> GSADAEYDVVVLGGGPGGYSAAFAAADEGLKVAIVERYKTLGGVCLNVGCIPSKALLHNAAVIDEVRHLAANGIKYPEPELDIDMLRAYKDGVVSRLTGGL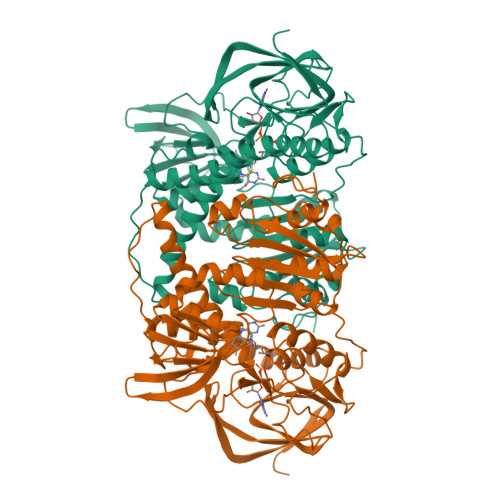AGMAKSRKVDVIQGDGQFLDPHHLEVSLTAGDAYEQAAPTGEKKIVAFKNCIIAAGSRVTKLPFIPEDPRIIDSSGALALKEVPGKLLIIGGGIIGLEMGTVYSTLGSRLDVVEMMDGLMQGADRDLVKVWQKQNEYRFDNIMVNTKTVAVEPKEDGVYVTFEGANAPKEPQRYDAVLVAAGRAPNGKLISAEKAGVAVTDRGFIEVDKQMRTNVPHIYAIGDIVGQPMLAHKAVHEGHVAAENCAGHKAYFDARVIPGVAYTSPEVAWVGETELSAKASARKITKANFPWAASGRAIANGCDKPFTKLIFDAETGRIIGGGIVGPNGGDMIGEVCLAIEMGCDAADIGKTIHPHPTLGESIGMAAEVALGTCTDLPPQKK> SNADVNPLTLGIETVGGVMTKLIGRNTVIPTKKSQVFSTAADSQSAVSIVIYEGERPMVMDNHKLGNFDVTGIPPAPRGVPQIEVTFEIDVNGILHVSAEDKGTGNK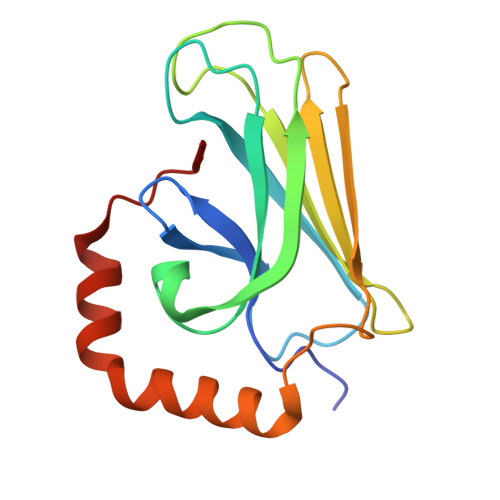NKLTITNDHNRLSPEDIERMINDADKFAADDQAQKEKVESRNELE>[2x]MSKLPFLSRAAFARITTPIARGLLRVGLTPDVVTILGTTASVAGALTLFPMGKLFAGACVVWFFVLFDMLDGAMARERGGGTRFGAVLDATCD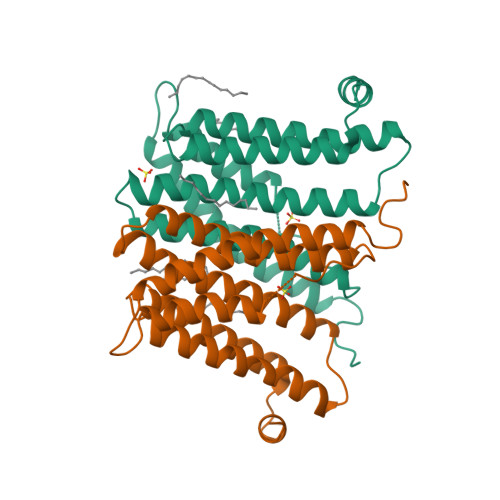RISDGAVFCGLLWWIAFHMRDRPLVIATLICLVTSQVISYIKARAEASGLRGDGGFIERPERLIIVLTGAGVSDFPFVPWPPALSVGMWLLAVASVITCVQRLHTVWTSPGAIDRMAIPGKGDR> MTIRNQRFSLLKEPISSTLNQHLIDYPTPSNLSYWWGFGSLAGICLVIQIVTGVFLAMHYTPHVDLAFNSVEHVMRDVEGGWLLRYMHANGASMF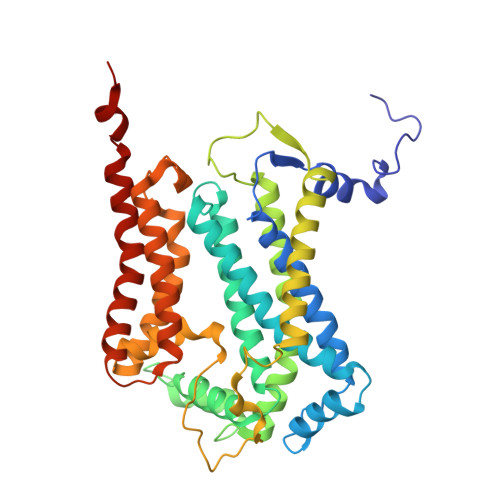FIVVYLHIFRGLYYASYSSPREFVWCLGVVIFLLMIVTAFTGYVLPWGQMSFWGATVITSLASAIPVVGDTIVTWLWGGFSVDNATLNRFFSLHYLLPFLLVGASLLHLAALHQYGSNNPLGVHSEMDQISFYPYFYVKDLVGWVAFAIFFSIWIFYAPNVLGHPDNYIPANPMSTPPHIVPEWYFLPIYAILRSIPDKSGGVAAIALVFICLLALPFFKSMYVRSSSFRPIYQGIFWLLLADCLLLGWIGCQPVEAPFVTIGQISSFVFFLFFAITPILGRVGRGIPNSYTTDETEM> 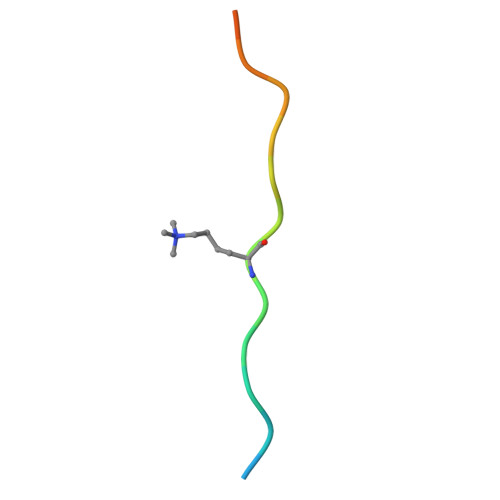LATKAARKSAPATGGVKK>[14x]MQQGQMAYDRAITVFSPDGRLFQVEYAREAVKKGSTALGMKFANGVLLISDKK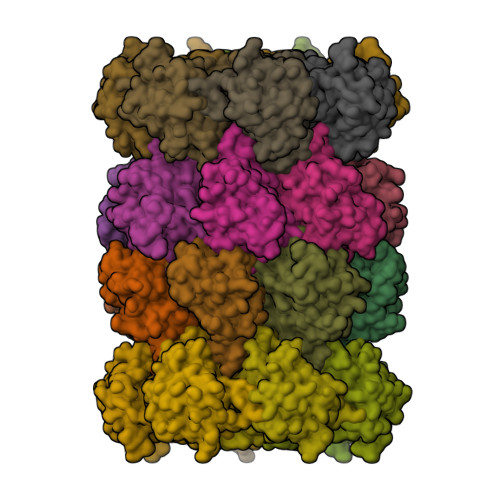VRSRLIEQNSIEKIQLIDDYVAAVTSGLVADARVLVDFARISAQQEKVTYGSLVNIENLVKRVADQMQQYTQYGGVRPYGVSLIFAGIDQIGPRLFDCDPAGTINEYKATAIGSGKDAVVSFLEREYKENLPEKEAVTLGIKALKSSLEEGEELKAPEIASITVGNKYRIYDQEEVKKFL;>[14x]MNQTLETGTTTVGITLKDAVIMATERRVTMENFIMHKNGKKLFQIDTYTGMTIAGLVGDAQVLVRYMKAELELYRLQRRVNMPIEAVATLLSNMLNQVKYMPYMVQLLVGGIDTAPHVFSIDAAGGSVEDIYASTGSGSPFVYGVLESQYSEKMTVDEGVDLVIRAISAAKQRDSASGGMIDVAVITRKDGYVQLPTDQIESRIRKLGLIL> HHLV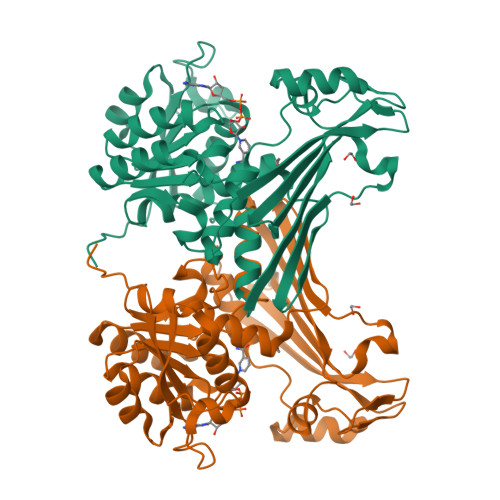PRGSYKVGIWGFGAMGSGIAKNILSKKNLKLVGVHDFREEYIEKDVGELLGLGKIGIKVYPDPITMVKQTDPDLVVIATNSFISVVKDQIISILKENKNVITIAEEMAFPFSKDPKAANEIDTVAKDHNVSVLGTGVNPGFVLDTLIITLTGICLNVQRIKAARINDLSPFGPTVMETQGVGTTPEEFKQGIKSGKIVGHIGFEQSIHMIAKALGWEIDRIEQKREPIISNVMRETKYVKVQPGMVAGCNHTAKAFYKNELLIELEHPQQVLPHLENVQTGDYITIQGDPDISMGINPEIPGGKGTIAIATNMIPSVVEARPGLLTMVDLPIPRALLAEVH>MTQELGNANFENFIGATEGFSEIAYQFTSHILTLGYAVMLAGLLYFILTIKNVDKKFQMSNILSAVVMVSAFLLLYAQAQNWTSSFTFNEEVGRYFLDPSGDLFNNGYRYLNWLIDVPMLLFQILFVVSLTTSKFSSVRNQFWFSGAMMIITGYIGQFYEVSNLTAFLVWGAISSAFFFHILWVMKKVINEGKEGISPAGQKILSNIWILFLISWTLYPGAYLMPYLTGVDGFLYSEDGVMARQLVYTIADVSSKVIYGVLLGNLAITLSKNKELVEANS[5x]

To address the challenges of cryo-EM/ET sample preparation, we developed EasyGrid, a fully automated and modular platform for high-throughput sample vitrification using ethane-jetting technology. EasyGrid is designed to provide fine control over sample preparation parameters and to perform automated grid quality control at cryogenic temperature. We demonstrated that it is suited for optimizing SPA grids by obtaining high resolution maps of three different macromolecular complexes (i.e. apoferritin, yeast ribosomes and pentamers of KR2 bacterial rhodopsin).

The EasyGrid SPA routine starts with enhancing the hydrophilicity of a grid using atmospheric plasma treatment, then dispensing the sample or a pre- coating solution on the grid in a user-designed pattern (typically a line of 100 droplets) using microfluidic nozzles ([Fig fig3]). A rapid sequence of sample spreading with the pressure-wave system followed by jet-vitrification allows freezing unstably thin sample films on grids ([Fig fig3], right panel) before storing them in cryo-boxes at LN_2_ temperature. We implemented SPA grid preparation protocols to study human apoferritin, yeast ribosomes, and bacterial KR2 rhodopsin samples ([Fig fig3]) and determined their structures at 1.9 Å, 2.4 Å, and 2.3 Å, respectively using conventional cryo-EM acquisition and processing schemes ([Fig figs2], [Fig figs3] and [Fig figs4]). The structure of the KR2 rhodopsin complex was not previously described with cryo-EM although a structure obtained at high salt concentrations with X-ray crystallography was already available. Our cryo-EM map at 2.3Å resolution shows key features of KR2 rhodopsin including the interprotomeric sodium binding site and the functional, expanded conformation of the central region of the pentamer with numerous water molecules populating the internal cavities. The cryo-EM map additionally reveals all 4 of the water molecules located in the Schiff base cavity of KR2 while only 3 water molecules were resolved in X-ray crystallography data at a comparable map resolution (2.2Å). Last, we observed a different organization of the hydrophobic tails of lipid molecules in the interprotomeric clefts compared to published crystal structures, suggesting the high flexibility of lipid-protein interactions in KR2 complexes ([Fig figs5]). Moreover, pressure-wave-based spreading did not prevent us from solving macromolecular structures at ∼2Å resolution, suggesting that EasyGrid is compatible with a majority of samples.> GESRDCHGTICHPVNEFCYVATERCHPCIEVCNNQTHNYDAF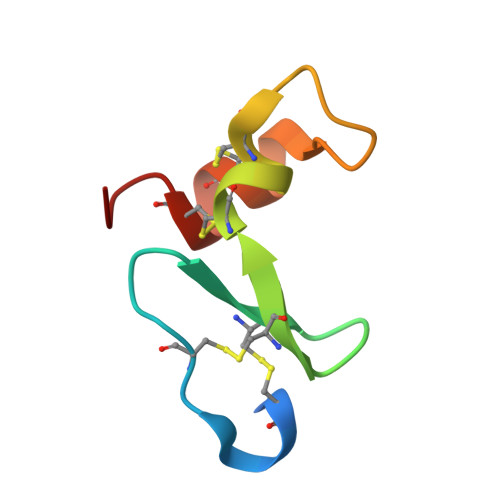LCAKECSAYK> MSTNKVNKERTFLAVKPDGVARGLVGEIIARYEKKGFVLVGLKQLVPTKDLAESHYAEHKERPFFGGLVSFITSGPVVAMVFEGKGVVASARLMIGV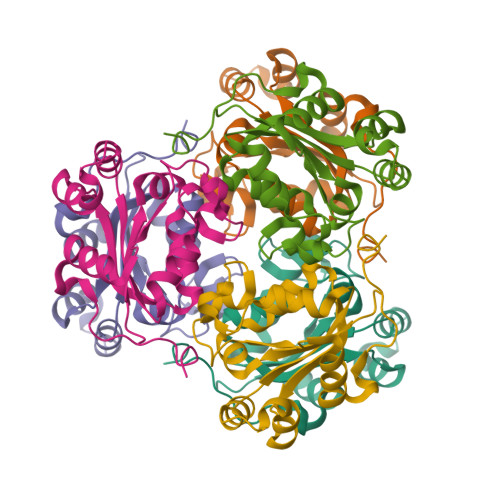TNPLASAPGSIRGDFGVDVGRNIIAGSDSVESANREIALWFKPEELLTEVKPNPNLYE>GSLKSACVVCL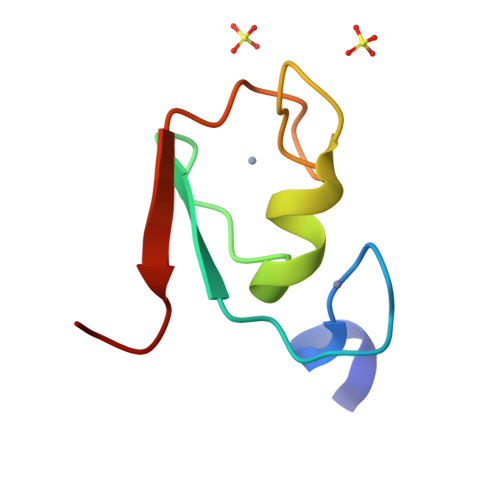SSFKSCVFLECGHVCSCTECYRALPEPKKCPICRQAITRVIPLYNS[6x]> LTAKHRPSVVWLHNAECTGCTEAAIRTIKPYIDALILDTISLDYQETIMAAAGEAAEAALHQALEGKDGYYLVVEGGLPTIDGGQWGMVAGHPMIETTKKAAAKAKGIICIGTCSAYGGVQKAKPNPSQAKGVSEALGVKTINIPGCPPNPINFVGAVVHVLTKGIPDLDENGRPKLFYGELVHDNCPR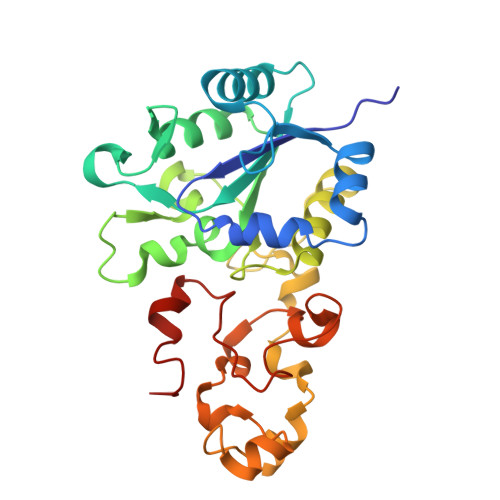LPHFEASEFAPSFDSEEAKKGFCLYELGCKGPVTYNNCPKVLFNQVNWPVQAGHPCLGCSEPDFWDTMTPFYEQG> IWLLQSLLRLGDEINAY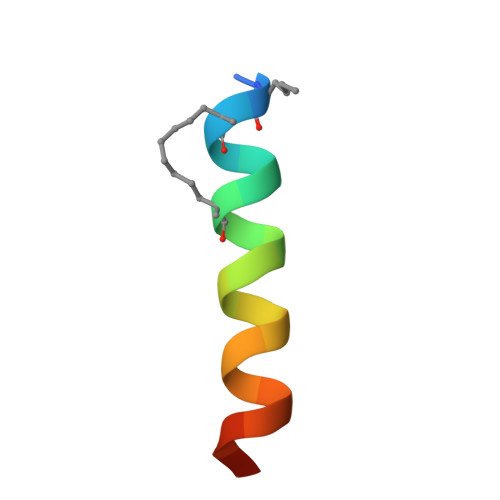YARRX> METQLQSIFEEVVKTEVIEEAFPGMFMDTPEDEKTKLISCLGAFRQFWGGLSQESHEQCIQWIVKFIHGQHSPKRISFLYDCLAMAVETGLLPPRLVCESLINSDTLEWERTQLWALTFKLVRKIIGGVDYKGVRDLLKVILEKILTIPNTVSSAVVQQLLAAREVIAYILERNACLLPAYFAVTEIRKLYPEGKLPHWLLGNLVSDFVDTFRPTARINSICGRCSLLPVVNNSGAICNSWKLDPATLRFPLKGLLPYDKDLFEPQTALLRYVLEQPYSRDMVCNMLGLNKQHKQRCPVLEDQLVDLVVYAMERSETEEKFDDGGTSQLLWQHLSSQLIFFVLFQFASFPHMVLSLHQKLAGRGLIKGRDHLMWVLLQFISGSIQKNALADFLPVMKLFDLLYPEKEYIPVPDINKPQSTHAFAMTCIWIHLNRKAQNDNSKLQIPIPHSLRLHHEFLQQSLRNKSLQMNDYKIALLCNAYSTNSECFTLPMGALVETIYGNGIMRIPLPGTNCMASGSITPLPMNLLDSLTVHAKMSLIHSIATRVIKLAHAKSSVALAPALVETYSRLLVYMEIESLGIKGFISQLLPTVFKSHAWGILHTLLEMFSYRMHHIQPHYRVQLLSHLHTLAAVAQTNQNQLHLCVESTALRLITALGSSEVQPQFTRFLSDPKTVLSAESEELNRALILTLARATHVTDFFTGSDSIQGTWCKDILQTIMSFTPHNWASHTLSCFPGPLQAFFKQNNVPQESRFNLKKNVEEEYRKWKSMSNENDIITHFSMQGSPPLFLCLLWKMLLETDHINQIGYRVLERIGARALVAHVRTFADFLVYEFSTSAGGQQLNKCIEILNDMVWKYNIVTLDRLILCLAMRSHEGNEAQVCYFIIQLLLLKPNDFRNRVSDFVKENSPEHWLQNDWHTKHMNYHKKYPEKLYFEGLAEQVDPPVQIQSPYLPIYFGNVCLRFLPVFDIVIHRFLELLPVSKSLETLLDHLGGLYKFHDRPVTYLYNTLHYYEMHLRDRAFLKRKLVHA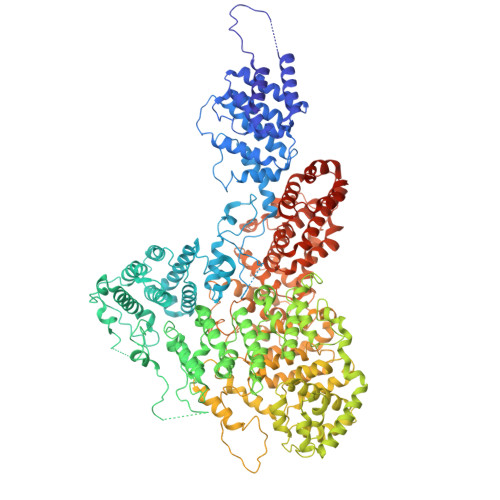IIGSLKDNRPQGWCLSDTYLKCAMNAREENPWVPDDTYYCRLIGRLVDTMAGKSPGPFPNCDWRFNEFPNPAAHALHVTCVELMALAVSGKEVGNALLNVVLKSQPLVPRENITAWMNAIGLIITALPEPYWIVLHDRIVSVISSPSLTSETEWVGYPFRLFDFTACHQSYSEMSCSYTLALAHAVWHHSSIGQLSLIPKFLTEVLLPIVKTEFQLLYVYHLVGPFLQRFQQERTRCMIEIGVAFYDMLLNVDQCSTHLNYMDPICDFLYHMKYMFTGDSVKEQVEKIICNLKPALKLRLRFITHISKMEPAAVPPQAMNSGSPAPQSNQVPVSLPVTQ> IVGGQECKDGECPWQA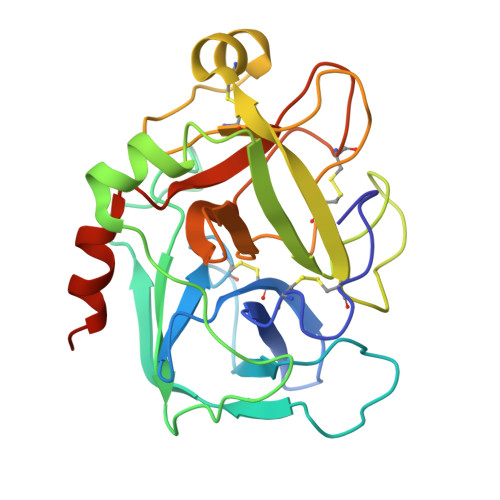LLINEENEGFCGGTILSEFYILTAAHCLYQAKRFKVRVGDRNTEQEEGGEAVHEVEVVIKHNRFTKETYDFDIAVLRLKTPITFRMNVAPACLPERDWAESTLMTQKTGIVSGFGRTHEKGRQSTRLKMLEVPYVDRNSCKLSSSFIITQNMFCAGYDTKQEDACQGDAGGPHVTRFKDTYFVTGIVSWGEGCARKGKYGIYTKVTAFLKWIDRSMKTRGLPKAK> GAMGSGEPQSP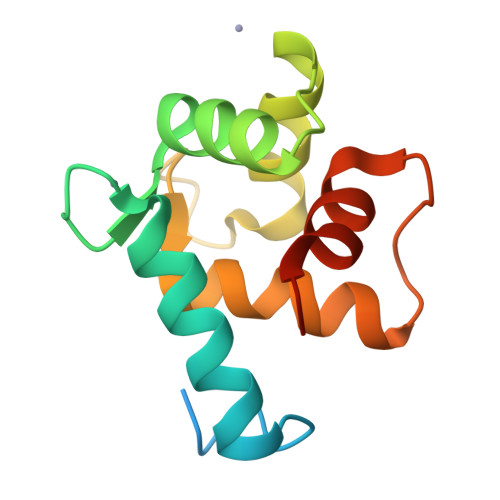SRRVFNPYTEFKEFSRKQIKDMEKMFKQYDAGRDGFIDLMELKLMMEKLGAPQTHLGLKNMIKEVDEDFDSKLSFREFLLIFRKAAAGELQEDSGLCVLARLSEIDVSS>[10x]GHMKKRKARSLLPLSTSLDHRSKEELHQDCL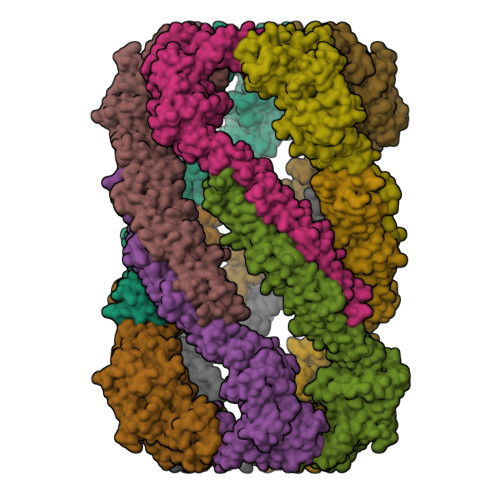VLATAKHSRELNEDVSADVEERFHLGLFTDRATLYRMIDIEGKGHLENGHPELFHQLMLWKGDLKGVLQTAAERGELTDNLVAMAPAAGYHVWLWAVEAFAKQLCFQDQYVKAASHLLSIHKVYEAVELLKSNHFYREAIAIAKARLRPEDPVLKDLYLSWGTVLERDGHYAVAAKCYLGATCAYDAAKVLAKKGDAASLRTAAELAAIVGEDELSASLALRCAQELLLANNWVGAQEALQLHESLQGQRLVFCLLELLSRHLEEKQLSEGKSSSSYHTWNTGTEGPFVERVTAVWKSIFSLDTPEQYQEAFQKLQNIKYPSATNNTPAKQLLLHICHDLTLAVLSQQMASWDEAVQALLRAVVRSYDSGSFTIMQEVYSAFLPDGCDHLRDKLGDHQSPATPAFKSLEAFFLYGRLYEFWWSLSRPCPNSSVWVRAGHRTLSVEPSQQLDTASTEETDPETSQPEPNRPSELDLRLTEEGERMLSTFKELFSEKHASLQNSQRTVAEVQETLAEMIRQHQKSQLCKSTANGPDKNEPEVEAEQPLCSSQSQCKEEKNEPLSLPELTKRLTEANQRMAKFPESIKAWPFPDVLECCLVLLLIRSHFPGCLAQEMQQQAQELLQKYGNTKTYRRHCQTFCM>[2x]GMNKKTQLL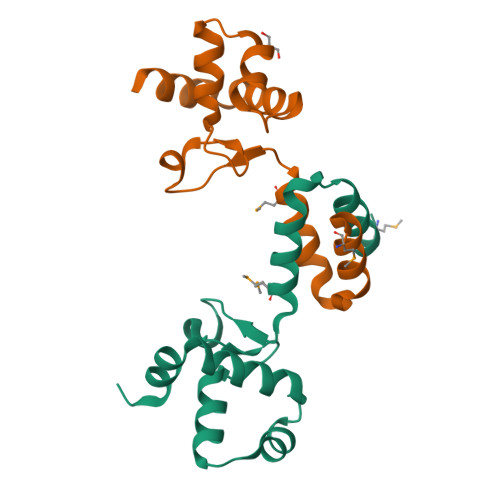EVIAALPEELVDQALNYVQMLQNPIQITPGVCGGQARIRNTRIPVWTLVAYRQQGAPDKELLANYPGLTAEDLSAAWHYYEQNPEQIDREIAQDDLV> MSKKRSYSDGDE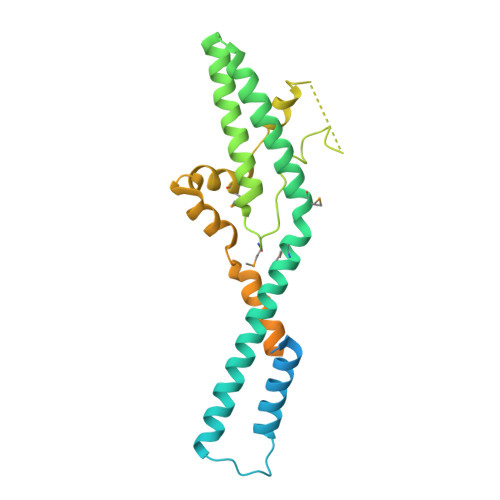ASGDSEVAAAKRQKINKAHFKKKRHHQNKSDEGKESLGAIKKRARAIERLLARDNLKLPANKQKELERELKAHKERIKDIEFKRERSKMISKYHMVRFFERRKALRFAQQLERRLSKATDPVEIAQLKADLHIAQVDIDYTKYFPFMEPYVSLYAQVRGNKEGDDKDGKDDKGAAARYLHAPRPPMWYEIEKIREEGVTALEKLQNRAPEKVIKKVDAKVEKPKKPSKDKDKRNGDDGKEKKKKERAEDTQDKQEWVGKKKEKEKKDKPKSGKGKKDESPARSESEESDSDGGFFEED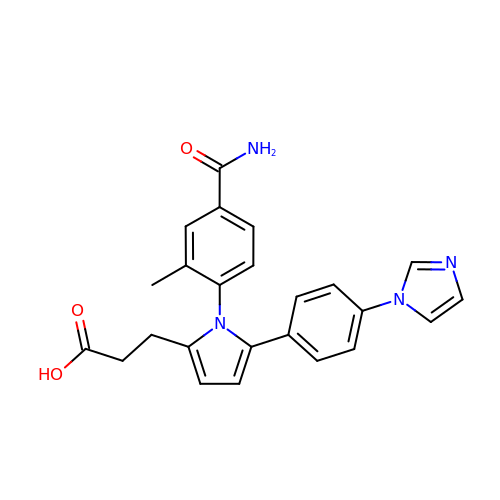3-{1-(4-carbamoyl-2-methylphenyl)-5-[4-(1H-imidazol-1-yl)phenyl]-1H-pyrrol-2-yl}propanoic acid | C24 H22 N4 O3 | YVPGZQLRPAGKLA-UHFFFAOYSA-N> SMGPCDIYEAGDTPCVAAHSTTRALYSSFSGALYQLQRGSDDTTTTISPLTAGG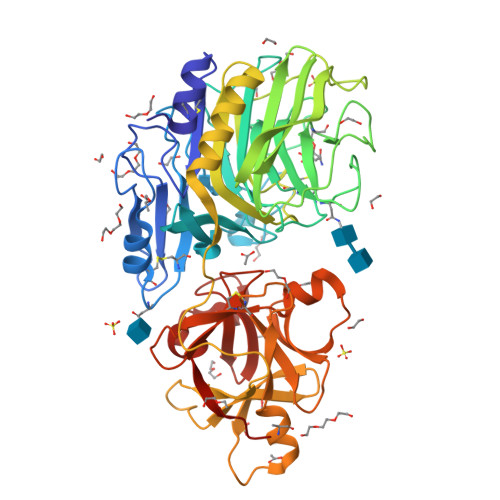IADASAQDTFCANTTCLITIIYDQSGNGNHLTQAPPGGFDGPDTDGYDNLASAIGAPVTLNGQKAYGVFMSPGTGYRNNEATGTATGDEAEGMYAVLDGTHYNDACCFDYGNAETSSTDTGAGHMEAIYLGNSTTWGYGAGDGPWIMVDMENNLFSGADEGYNSGDPSISYRFVTAAVKGGADKWAIRGANAASGSLSTYYSGARPDYSGYNPMSKEGAIILGIGGDNSNGAQGTFYEGVMTSGYPSDDTENSVQENIVAAKYVVGSLVSGPSFTSGEVVSLRVTTPGYTTRYIAHTDTTVNTQVVDDDSSTTLKEEASWTVVTGLANSQCFSFESVDTPGSYIRHYNFELLLNANDGTKQFHEDATFCPQAALNGEGTSLRSWSYPTRYFRHYENVLYAASNGGVQTFDSKTSFNNDVSFEIETAFAS>MVSVSPSKVTLPRGGSVLVTCSASCDQPKLLGIETPLVKKELLLPGNNRKVYELSNVQEDSQVMCYANCPDGQSTAKAFLTVYWT[14x];>[14x]MNVDLVFLFDGSMSLQP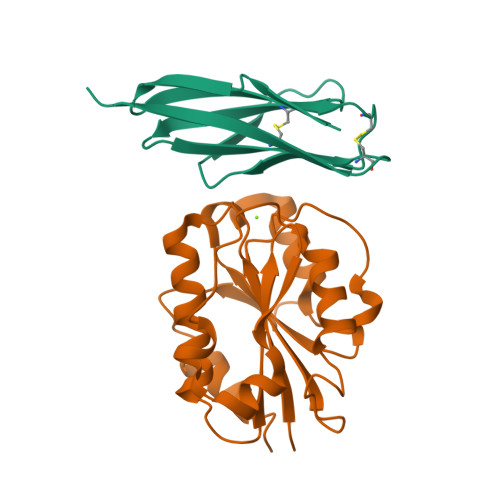DEFQKILDFMKDVMKKLSNTSYQFAAVQFSTSYKTEFDFSDYVKWKDPDALLKHVKHMLLLTNTFGAINYVATEVFREELGARPDATKVLIIITDGEATDSGNIDAAKDIIRYIIGIGKHSQTKESQETLHKFASKPASEFVKILDTFEKLKDLFTELQKKIY> MSIQHFRVALIPFFAAFCLPVFAHPETLVKVKDAEDQLGARVGYIELDLNSGKILESFRPEERFPMMXTFKVLLCGAVLSRIDAGQEQLGRRIHYSQNDLVEYSPVTEKHLTDGMTVRELCSAAITM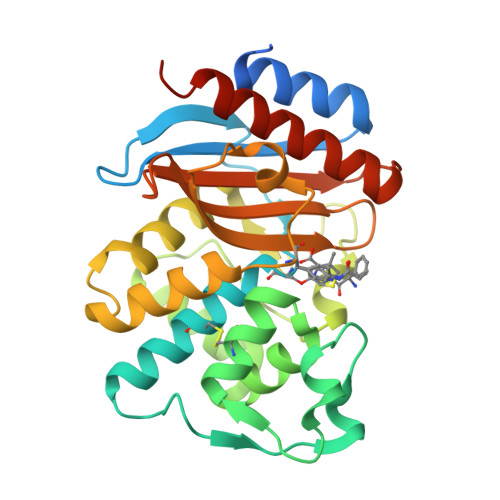SDNTAANLLLTTIGGPKELTAFLHNMGDHVTRLDRWNPELNEAIPNDERDTTMPVAMATTLRKLLTGELLTLASRQQLIDWMEADKXAGPLLRSALPAGWFIADKSGAGERGSRGIIAALGPDGKPSRIVVIYTTGSQATMDERNRQIAEIGASLIKHWAAALEHHHHHH> MSSQIRQNYSTDVEAAVNSLVNLYLQASYTYLSLGFYFDRDDVALEGVSHFFRE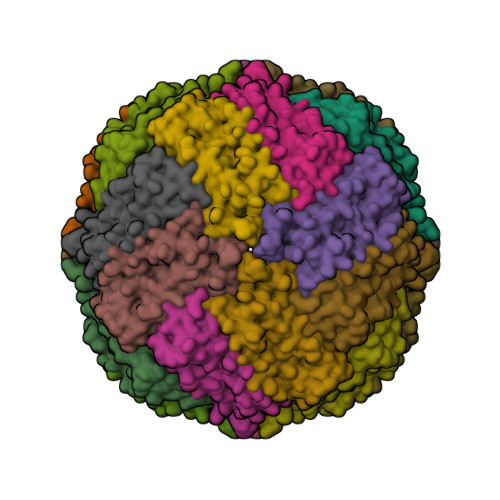LAAAKRAGYERLLKMQNQRGGRALFQDIKKPAEDEWGKTPDAMKAAMALEKKLNQALLDLHALGSARTDPHLCDFLETHFLDEEVKLIKKMGDHLTNLHRLGGPEAGLGEYLFERLTLKHD> SNADPKEGVQYEVLSTSLENDGMAPVTEVFALSCGHCRNMENFLPVISQEAGTDIGKMHITFNQSAHIASMFYYAAEMQVDGAPDHAFMEDLFAATQMGEGTTLTEQQEAYSKAFTSRGLVSPYDFNEEQR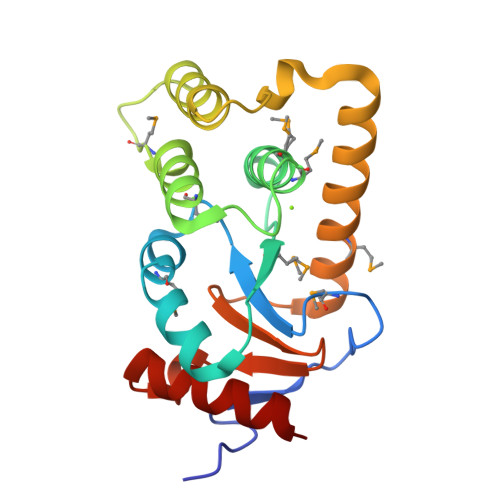DTLIKKVDNAKMLSEKSGISSVPTFVVNGKYNVLIGGHDDPKQIADTIRYLLEK> KIRRLKQKNARLKQEIAA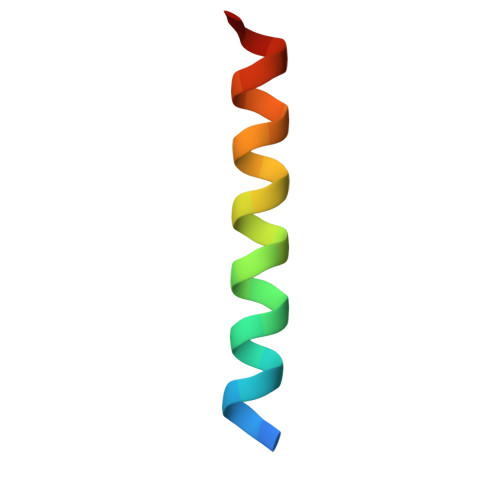LEYEIAALEQ>[2x]SFGSDVRPAAAQEVVGGGDLGPNVLVFDPSTPDIQGKVDEVFRKQESNQFGTDRYALMFKPGTYNDINAQIGFYTSIAGLGLNPDDTTFNGDVTVDAGWFDGNATQNFWRSAENLALNPVNGTNRWAVSQAAPFRRMHVKGGLNLAPDGYGWASGGYIADSKIDGEVGPYSQQQWYTRDSSVGGWGNGVWNMTFSGVEGAPAQSFPEPPYTTLETTPVSREKPFLYLDGDDYKVFVPAKRTNARGTSWGNGTPEGESLPLDQFYVVKPGATAETINAAVDQGLHLLFTPGVYHVDQPIEIDRANTVALGLGLATIIPDNGVTALKVGDVDGVKVAGLLVDAGPVNSETLVEVGSDGASGDHAANPTS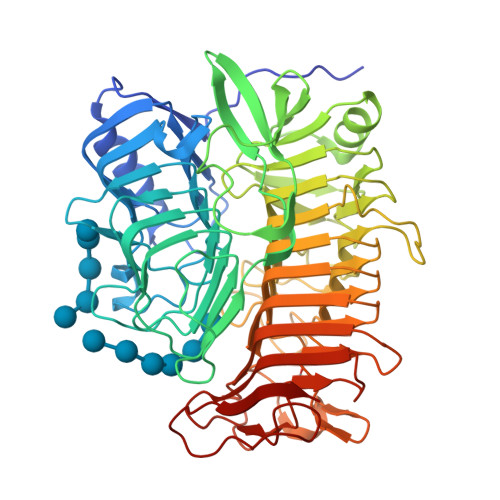LQDVFVRIGGAGPGKATTSIVVNSNDTIIDHTWVWRADHGEGVGWETNRADYGVHVKGDNVLATGLFVEHFNKYDVQWSGENGKTIFYQNAKAYDAPDQAAIQNGDIKGYAAYKVDDSVTTHEGWGMGSYCYFNVNPDIRQQHGFQAPVKPGVKFHDLLVVSLGGKGQYEHVINDIGDPTSGDTTIPSQVVSFP> GSDTSGILLASITGAGSAFQAYAGCYLTAFRNDPRTLTLRMDKTRGERISNVLVILSGGALSHAVEEVVQIAPGAVRNLATLGASTVQFLHNFRS

Plant pathogens secrete proteins, known as effectors, that function in the apoplast or inside plant cells to promote virulence. Previous studies of Fol-infected tomato identified a number of fungal proteins within the xylem sap. These secreted in xylem (SIX) effector proteins represent major pathogenicity determinants across different formae speciales of F. oxysporum. Currently, 14 SIX effectors have been identified in Fol consisting of small (less than 300 amino acids in length), secreted, cysteine-rich proteins. Here, we demonstrate that despite their sequence diversity, the Fol SIX effectors can be classified into a reduced set of structural families.

Avr2, a member of the ToxA-like effector family, exhibited structural similarity with the SIX7 and SIX8 models (Z-scores > 5). Analysis of the models and topology show that SIX7 and SIX8 both consist of a β-sandwich fold, strongly indicating their inclusion within the ToxA-like structural family. Here we demonstrate that both protein pairs contain a ToxA-like family member (Avr2, SIX8) and a structural family 4 member (SIX5, PSL1). Likewise, SIX8 and PSL1 are adjacent divergently transcribed genes in the Fol genome, and we demonstrate here a physical interaction between the proteins. We subsequently utilised AlphaFold2-Multimer through ColabFold to model the interaction. Manual inspection of the top 5 models (top model shown in Figure 4C) demonstrated that the thiol side chain of a free cysteine in PSL1 (Cys 37) and SIX8 (Cys 58) co-localised in the dimer interface, suggesting that an inter-disulfide bond may mediate the interaction. Collectively, these data demonstrated that the SIX8-PSL1 heterodimer is mediated via a disulfide bond. We crystallised and solved the structure of SIX8_C58S at 1.28 Å which confirms its inclusion within the ToxA-like structural family. Despite this, AlphaFold2 models were critical in solving the structure of SIX6 and SIX8 as templates for molecular replacement. When the modelling was repeated with the SIX8C58S experimentally derived structure included as a template, the interaction models and heterodimer interface were of higher quality and essentially identical. The region of SIX8 involved in the interaction with PSL1 was modelled incorrectly by AlphaFold2 when compared to the structure.> MKAKRVPGGKELLLDLDAPIWAGAESTTFEMFPTPLVMVKEVSPFLALSEGHGVIKRLDVAALHNGSMIALRLKWASEKHDKIVDLNSFVDGVGAMFPVARGAQAVTMGATGRPVNAWYWKANANEPMEIVAEGFSAVRRMKDKAGSDLKAVAQHRNGEWNVILCRSMATGDG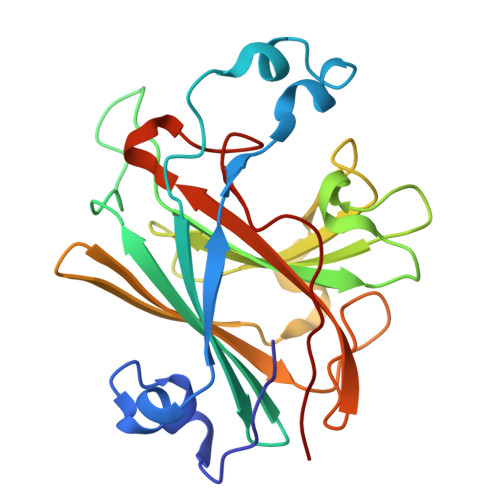LAKLQAGGSSKIAFAVWSGGNAERSGRKSYSGEFVDFEILK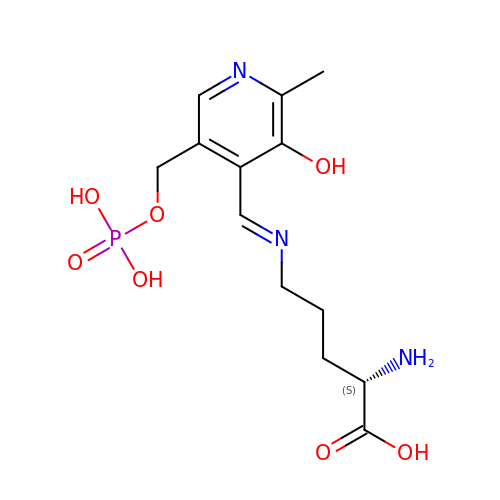(E)-N~5~-({3-hydroxy-2-methyl-5-[(phosphonooxy)methyl]pyridin-4-yl}methylidene)-L-ornithine | C13 H20 N3 O7 P | RMKYDMCVWSLEGI-DMSFABOWSA-N>[3x]MRGSHHHHHHTAPHASSVPLEWPLSSQSGSYELR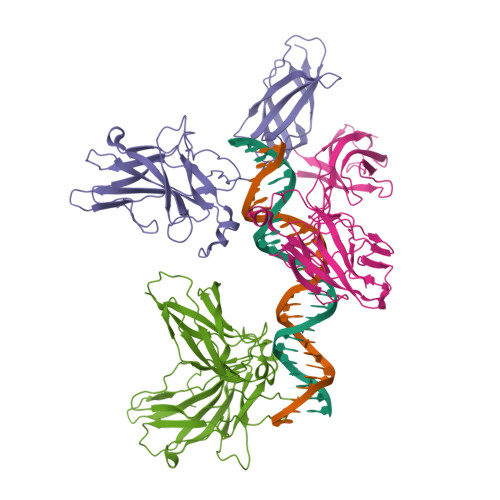IEVQPKPHHRAHYETEGSRGAVKAPTGGHPVVQLHGYMENKPLGLQIFIGTADERILKPHAFYQVHRITGKTVTTTSYEKIVGNTKVLEIPLEPKNNMRATIDCAGILKLRNADIELRKGETDIGRKNTRVRLVFRVHIPESSGRIVSLQTASNPIECSQRSAHELPMVERQDTDSCLVYGGQQMILTGQNFTSESKVVFTEKTTDGQQIWEMEATVDKDKSQPNMLFVEIPEYRNKHIRTPVKVNFYVINGKRKRSQPQHFTYHPV>[2x]GSAMGSSSHAPTEPDIQKDKDDSIIRENENIPAPLGTVVQLLFGS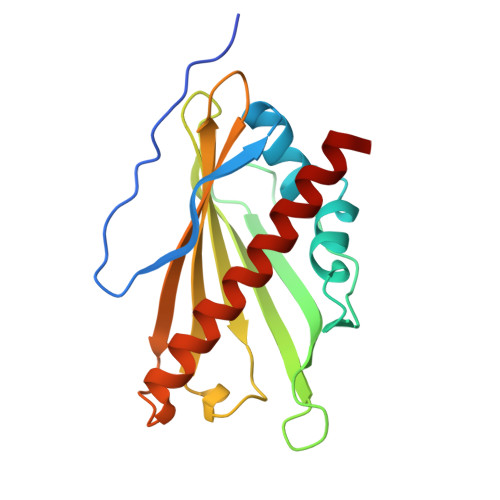NTEYMQKVITRDKNNVNVETIPKFTPSLVEGGSRHYEYTKKLNNSIGPKQTKCLLTESIEHMDINNYVLVTQTTKTPDVPSGSNFAVESKIFLFWGQHDTTNMTVITKINWTSKSFLKGAIEKGSVEGQKVSVDYMLSELRDIISR>[2x]SEEAKPATTTTIKNTKPQCRPEDYATRLQDLRVTFHRVKPTLQREDDYSVWLDGTVVKGCWGCSVMDWLLRRYLEIVFPAGDHVYPGLKTELHSMRSTLESIYKDMRQCPLLGCGDKSVISRLSQEAERKSDNGTRKGLSELDTLFSRLEEYLHSRK;>HGTELPSPPSVWFEAEFFHHILHWTPIPQQSESTCYEVALLRYGIESWNSISQCS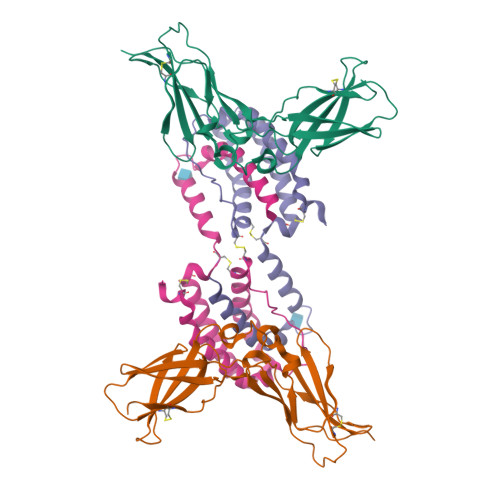QTLSYDLTAVTLDLYHSNGYRARVRAVDGSRHSQWTVTNTRFSVDEVTLTVGSVNLEIHNGFILGKIQLPRPKMAPAQDTYESIFSHFREYEIAIRKVPGQFTFTHKKVKHEQFSLLTSGEVGEFCVQVKPSVASRSNKGMWSKEECISLTRQYFTVTN[2x]>MTQVAEIKSPHEQRLEDNIAGKEDIYRESHKRVFKLLERFDGQKPAIDVERALYFTQSMAETVGQPLVLRWAKALMNVAKNITVMVQDDQLLLGRCGGHDGRYGILYPELDGDFLDIAVRDLPTRPQSPASISPEDAKIVVEQIAPFWKGRTYHEALNKALPAEVHKLTYDDPDGLISRFIVNETSSFRSSIQWVHDYEVVLKRGFNGLKQEMEEKLAALDPASPVDQVDKRPFIEATILVCDAIVLWAKRHADAARKAAEACADPVRKAELIRMAENAEHVPANPARDFYEAVQSQYFTQMFSRLEQKTGTTISNGRMDQYFYPFYKKDMEAGILTDEKTLEYLECMWVGMAEFIDMYISPAGGAFNEGYAHWEAVTIGGQTPDGRDATNDLTYLFLKSKREFPLHYPDLAARIHSRAPERYLWDVAETIKFGSGFPKLCNDEECIPLYVSKGATFEEALDYAVSGCIEIRMPNRDTYTSGGAYTNFASAVEMALYDGKMKKYGDVQLGIQTGDARKFKSWDEFWNAYVQQHMLLLRTTFIQQYIVIQTRAKHFAQPMGSVLHALCRKHCIDLHQPQIPEGLNFGYFEFMGLGTVIDSLAAIKKLVFEDKKLTMDQLIDALEANFEGYEDIQQLLRTAPCYGNDDEYADEIGRELDRMAVSFAAKYGKEMGINNDARYVPFTSHVPFGKVVSATPNGRVAWFPLADGSSPSHGADHNGPTAILLSNHNTKNYGMRARAARLINVKFTPKCVEGDAGTEKLVQFIRTWCDLKLWHIQFNVINADTLKKAQKDPQKYRNLIVRIAGYSAYFVDLTPDLQNDLIARTGHDQM[4x]

Desulfonation of isethionate by the bacterial glycyl radical enzyme (GRE) isethionate sulfite-lyase (IslA) generates sulfite, a substrate for respiration that in turn produces the disease-associated metabolite hydrogen sulfide. IslA belongs to the glycyl radical enzyme (GRE) superfamily, which performs diverse chemical reactions under anaerobic conditions (Backman et al., 2017). As is the case for the core architecture of all characterized GRE eliminases (Backman et al., 2017), IslA is dimeric with each monomer having a buried active site located centrally within a barrel comprised of two five-stranded half β barrels, anti-parallel to each other (β1–10), and surrounded by α helices. Gly805 and Cys468 are 5.2 Å from each other, competent for radical transfer from Gly805 to Cys468, and for the generation of a transient thiyl radical that initiates catalysis on the substrate.

Here, we present a 2.7 Å resolution X-ray structure of wild-type IslA from Bilophila wadsworthia with isethionate bound. After dialysis of the purified protein and increasing the isethionate concentration, a second IslA structure with the substrate Ise bound was obtained. In the active site of the second IslA structure, electron density was observed for the substrate Ise. A Glu residue (Glu470) hydrogen bonds with the hydroxyl group of Ise with an additional hydrogen bond being provided by the amide of Cys468. Several polar and electrostatic residues stabilize the negatively charged sulfonate group of Ise: Arg189 and Gln193 of β1, as well as Arg678 of β8, all of which are conserved in IslA homologs but not in other GREs according to sequence alignments performed using Clustal Omega. A water molecule that is present in all four molecules of the asymmetric unit provides another hydrogen bonding partner to the sulfonate group. Specificity in GREs is thus determined both by the substitution of residues on similarly positioned parts of β strands and by the active site alterations created by β strands repositioning. The biggest rearrangement of a β strand in IslA is found in β6, which allows Ise to bind in a much higher up position in the active site than those of Hyp or choline in their respective enzymes (see above). To secure Ise in this “higher” substrate-binding position, Arg678 extends into the active site from a position on β8 too distant to interact with substrate in CutC and HypD. Another difference generated by the unique Ise positioning is that the pro-R hydrogen of C2, rather than the pro-S hydrogen, is closer to the thiol of Cys468, with distances of 2.6 and 4.2 Å, respectively. Attempts to re-position Ise such that the pro-S hydrogen of C2 is closer to Cys468 result in a poor fit to the electron density.> IVGGQECKDGECPWQALLINEENEGFCGGTILSEFYILTAAHCLYQAKRFKVRVGDRNTEQEEGGEAVHEVEVVIKHNRFTKETYDFDIAVLRLKTPITFRMNVAPACLPERDWAESTLMTQKTGIVSGFGRTHEKGEQSTRLKMLEVPYVDRNSCKLSSSFIITQNMFCAGYDTKQEDACQGDSGGPHVTRFKDTYFVTGIVSWGEGCARKGKYGIYTKVTAFLKWIDRSMKTR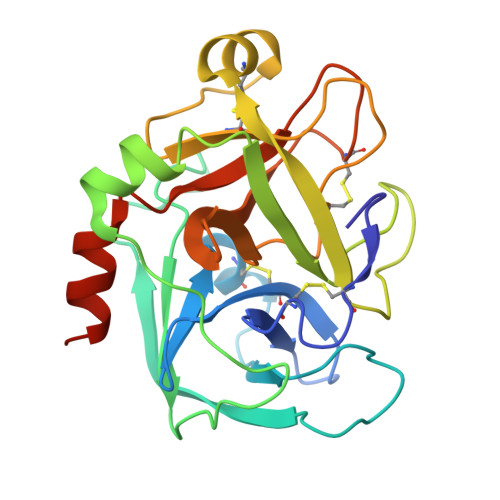GLPKAK>MELIRIAMKKDLENDNSLMNKWATVAGLKNPNPLYDFLNHDGKTFNEFSSIVNIVKSQYPDREYELMKDYCLNLDVKTKAARSALEYADANMFFEIEDVLIDSMISCSNMKSKEYGKVYKIHRELSNSVITEFEAVKRLGKLNIKTPEMNSFSRLLLLYHYLSTGNFSPMAQLIKQIDLSEISENMYIRNTYQTRVHVLMSNIKLNENSLEECREYSKKALESTNILRFQVFSYLTIGNSLLFSNYELAQENFLKGLSISVQNENYNMIFQQALCFLNNVWRKENKWINFESDSIMDLQEQAHCFINFNENSKAKEVLDKLDLLVHNDNELAMHYYLKGRLEQNKACFYS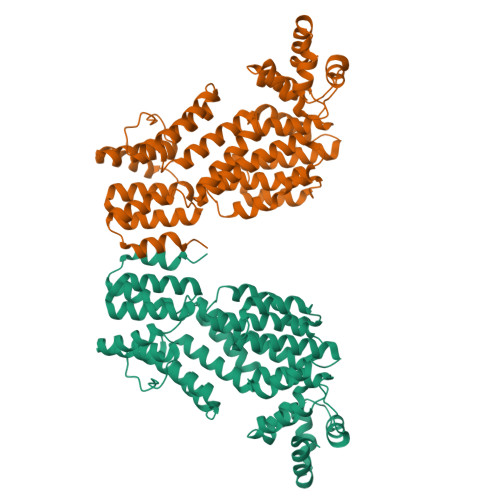SIEYFKKSNDKFLIRLPLLELQKMGENQKLLELLLLLEYA[2x]>[2x]GMSRKKNPSVIQFEKAITEKNYEAACTELLDILNKIDTNFGDIEGIDFDYPQQLETLMQDRIVYFCTRMSNAITQLFCDPQFSLSESGANRFFVVQRWLNLIFASSPYINADHILQTYNCNPERDSIYDIYLEPNKNVLMKFAVLYLPESNVNLNLDTMWETDKNICGSLCFALQSPRFIGTPAAFSKRSTILQWFPA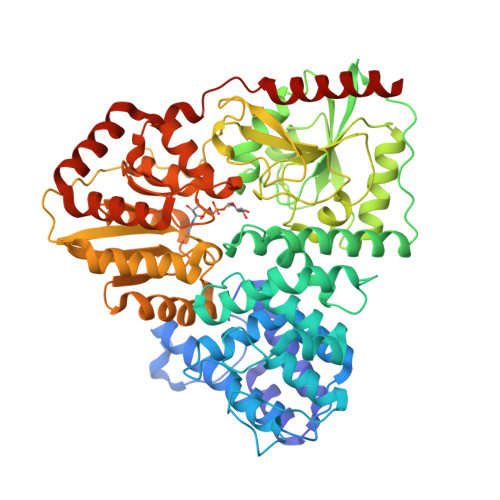KLEQFHVLDDLPSNISHDVYMHCSYDTAENKHNVKKALNQVIRSHLLKCGWQDRQITQIGMRNGKPVMVVVLEHFHSSHSIYRTHSTSMIAAREQFYLIGLGNNAVDQAGRDVFDEFHEFDGSNILKKLAFLKEMCEKNDAAVLYMPSIGMDLATIFVSNARFAPIQVIALGHPATTHSEFIEYVIVEDDYVGSESCFSETLLRLPKDALPYVPSSLAPTDVQYVLRETPEVVNIGIAATTMKLNPYFLETLKTIRDRAKVKVHFHFALGQSIGITHPYVARFIRSYLGDDATAHPHSPYNRYLDILHNCDMMLNPFPFGNTNGIIDMVTLGLVGVCKTGPEVHEHIDEGLFKRLGLPEWLIADSVEDYIERAIRLAENHQERLALRRHIIENNGLKTLFSGDPSPMGKTLFAKLTEWRQTNGI> MTTLTLSEAAPLLKKEFREGRLIPFLGAGFSKPLKLPDGSQLIASLAKTL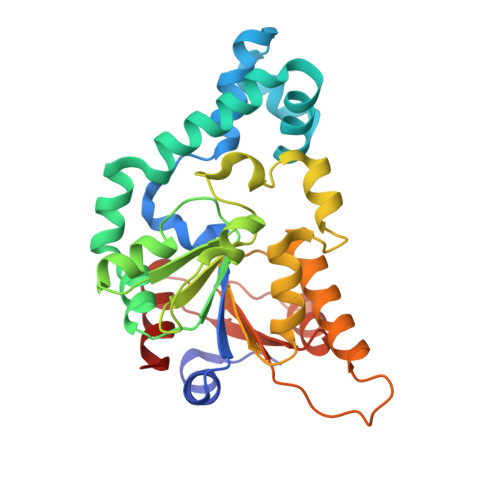GFEPELFDMHGRFEQLAEFFAISAPNRLQRLVYEMSLSFDSAEAEALREKSPMHRALAALDWRTIYTTNYDKHVEGALRDAGKQAAVLASFADFQGPRARDVCEVIKFHGTLDQPDTIVLTESSYFQRMALDAPPDQRLRADLLANSFLFIGYSFSDTNIRYIWYRMNQLREQSQLGVKHSQARRCFFATHGAGLVQPDILQQWNIDVIQLDPTDKSASVARLLESIA> GSKLIHVPKEDNSKEVTLDSLLEEGVLDKEIHKAITRMEFPGLTPVQQKTIKPILSSEDHDVIARAKTGTGKTFAFLIPIFQHLINTKFDSQYMVKAVIVAPTRDLALQIEAEVKKIHDMNYGLKKYACVSLVGGTDFRAAMNKMNKLRPNIVIATPGRLIDVLEKYSNKFFRFVDYKVLDEADR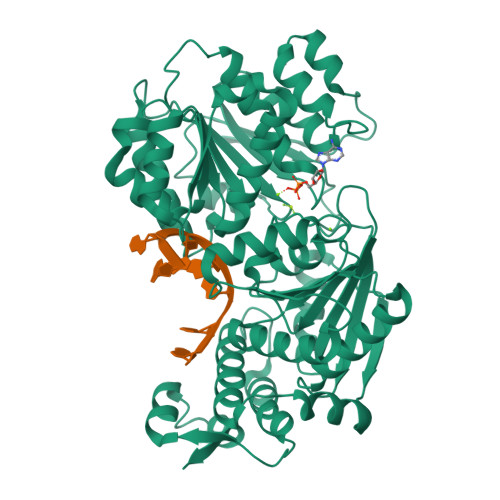LLEIGFRDDLETISGILNEKNSKSADNIKTLLFSATLDDKVQKLANNIMNKKECLFLDTVDKNEPEAHERIDQSVVISEKFANSIFAAVEHIKKQIKERDSNYKAIIFAPTVKFTSFLCSILKNEFKKDLPILEFHGKITQNKRTSLVKRFKKDESGILVCTDVGARGMDFPNVHEVLQIGVPSELANYIHRIGRTARSGKEGSSVLFICKDELPFVRELEDAKNIVIAKQEKYEPSEEIKSEVLEAVTEEPEDISDIVISLISSYRSCIKEYRFSERRILPEIASTYGVLLNDPQLKIPVSRRFLDKLGLSRSPIGKAMFEIR> SNAAASKKEIIVATNGSPRPFIYEENGELTGYEIEVVRAIFKDSDKYDVKFEKTEWSGVFAGLDADRYNMAVNNLSYTKERAEKYLYAAPIAQNPNVLVVKKDDSSIKSLDDIGGKSTEVVQATTSAKQLEAYNAEHTDNPTILNYTKADFQQIMVRLSDGQ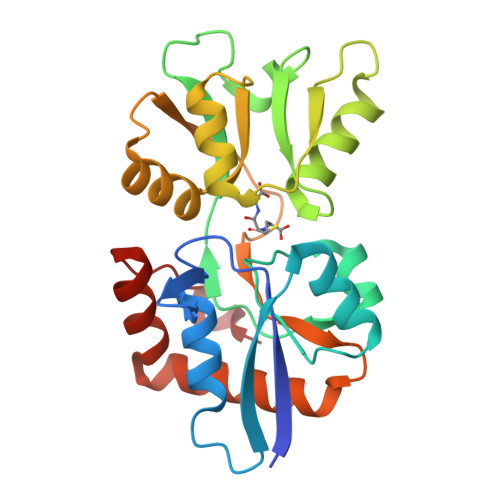FDYKIFDKIGVETVIKNQGLDNLKVIELPSDQQPYVYPLLAQGQDELKSFVDKRIKELYKDGTLEKLSKQFFGDTYLPAEADIK> MRSFLNLNSIPNVAAGNSCSIKLPIGQTYEVIDLRYSGVTPSQIKNVRVELDGRLLSTYKTLNDLILENTRHKRKIKAGVVSFHFVRPEM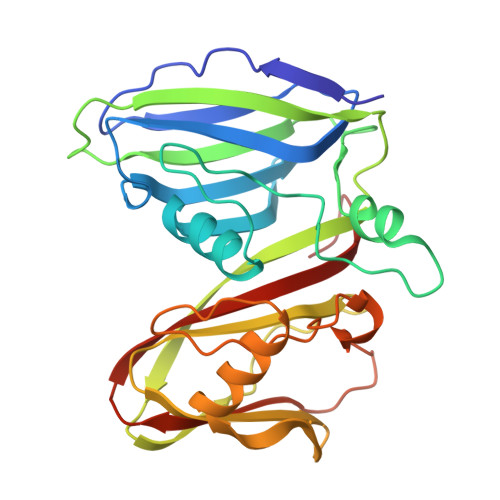KGVNVTDLVQQRMFALGTVGLTTCEIKFDIDEAAAGPKLSAIAQKSVGTAPSWLTMRRNFFKQLNNGTTEIADLPRPVGYRIAAIHIKAAGVDAVEFQIDGTKWRDLLKKADNDYILEQYGKAVLDNTYTIDFMLEGDVYQSVLLDQMIQDLRLKIDSTMDEQAEIIVEYMGVWSRNGF> GAGCAGACCAG;> AC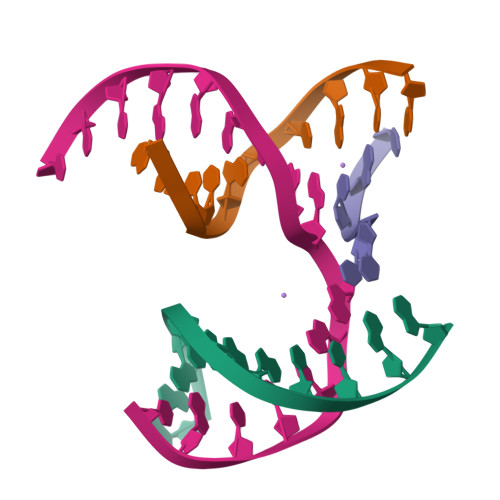ACCACTCA;> CTTGT;> TCTGAGTGGGGTCTGC> XGKVTFPKMKIPKFTFSGR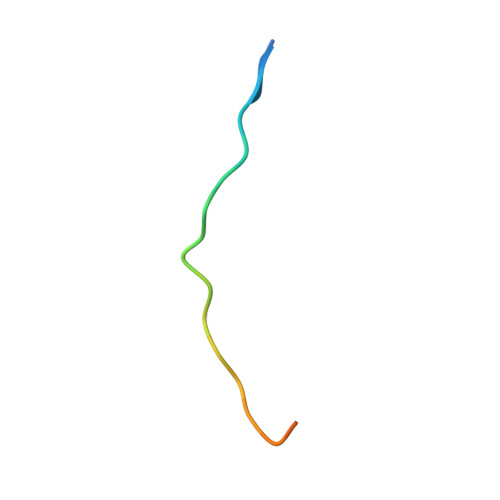ELX> ASMTGGQQMGAPITAYAQQTRGLLGCIITSLTGRDKNQVEGEVQIVSTATQTFLATCINGVCWTVYHGAGTRTIASPKGPVIQMYTNVDQDLVGWPAPQGSRSLTPCTCGSSDLYLVTRHADVIPVRRRGDSRGSLLSPRPISYLKGSSGGPLLCPAGHAVGLFRAAVCTRGVAKAVDFIPVENLET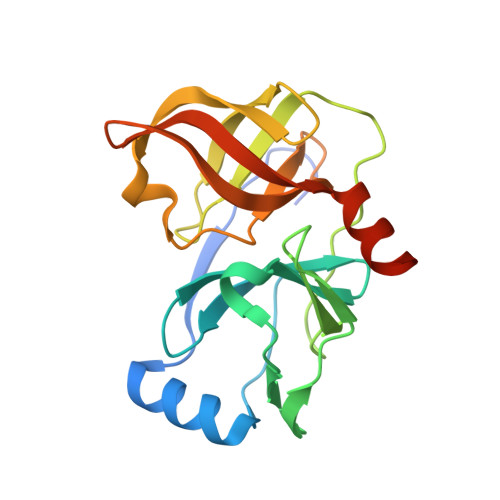TMRSGSHHHHHH>[6x]MKENKLDYIPEPMDLSLVDLPESLIQLSERIA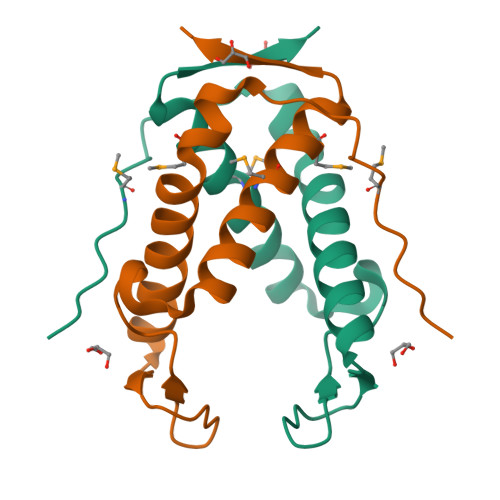ENVHEVAAKARIDEGWTYGEKRDDIHKKHPCLVPYDELPEEEKEADRNTAMNTIKMVKKLGFRIEKED1,1,1,3,3,3-hexafluoropropan-2-ol 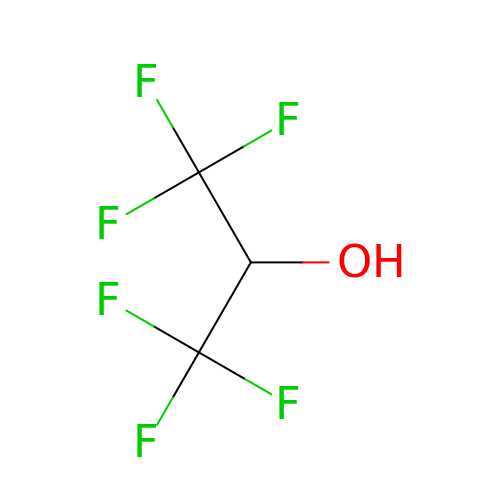| C3 H2 F6 O | BYEAHWXPCBROCE-UHFFFAOYSA-N> GIFAFENEQSSTVAPAKLYKALTKDSDEIVPKVIEPIQSVEIVEGNGGPGTIKKIIAIHDGHTSFVLHK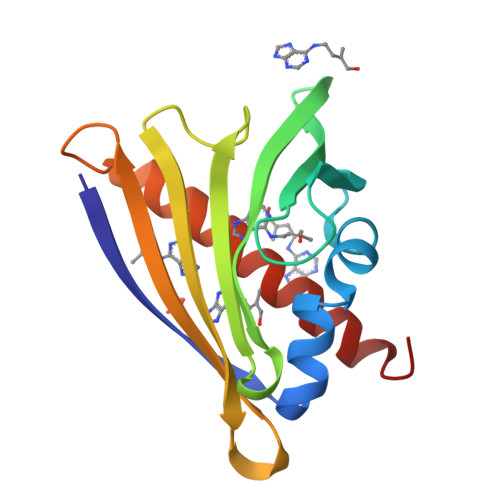LDAIDEANLTYNYSIIGGEGLDESLEKISYESKILPGPDGGSIGKINVKFHTKGDVLSETVRDQAKFKGLGLFKAIEGYVLAHPDY>[10x]MLFGRLTERAQRVLAHAQEEAIRLNHSNIGTEHLLLGLMKEPEGIAAKVLESFNITEDKVIEEVEKLIGHGQDHVGTLHYTPRAKKVIELSMDEAR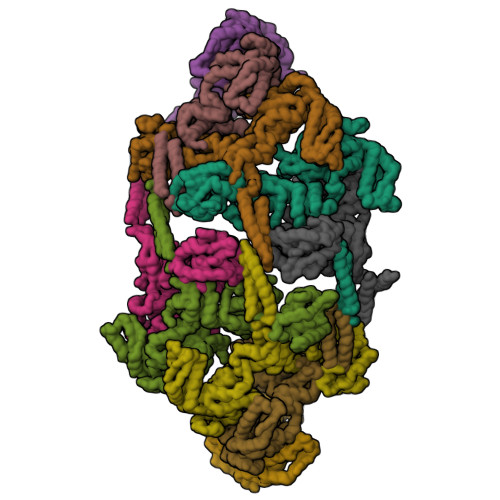KLHHNFVGTEHILLGLIRENEGVAARVFANLDLNITKARAQVVKALGNPEMSNKNAQASKSNNTPTLDSLARDLTVIAKDGTLDPVIGRDKEITRVIEVLSRRTKNNPVLIGEPGVGKTAIAEGLAQAIVNNEVPETLKDKRVMSLDMGTVVAGTKYRGEFEERLKKVMEEIQQAGNVILFIDELHTLVGAGGAEGAIDASNILKPALARGELQCIGATTLDEYRKNIEKDAALERRFQPVQVDEPSVVDTVAILKGLRDRYEAHHRINISDEAIEAAVKLSNRYVSDRFLPDKAIDLIDEASSKVRLKSHTTPNNLKEIEQEIEKVKNEKDAAVHAQEFENAANLRDKQTKLEKQYEEAKNEWKNTQNGMSTSLSEEDIAEVIAGWTGIPLTKINETESEKLLSLEDTLHERVIGQKDAVNSISKAVRRARAGLKDPKRPIGSFIFLGPTGVGKTELARALAESMFGDDDAMIRVDMSEFMEKHAVSRLVGAPPGYVGHDDGGQLTEKVRRKPYSVILFDEIEKAHPDVFNILLQVLDDGHLTDTKGRTVDFRNTIIIMTSNVGAQELQDQRFAGFGGSSDGQDYETIRKTMLKELKNSFRPEFLNRVDDIIVFHKLTKEELKEIVTMMVNKLTNRLSEQNINIIVTDKAKDKIAEEGYDPEYGARPLIRAIQKTIEDNLSELILDGNQIEGKKVTVDHDGKEFKYDIAEQTSETKTPSQA> MHQVDPNLTRRKGRLAALAIAAMASASLVTVAVPATANADPEPAPPVPTTAASPPSTAAAPPAPATPVAPPPPAAANTPNAQPGDPNAAPPPADPNAPPPPVI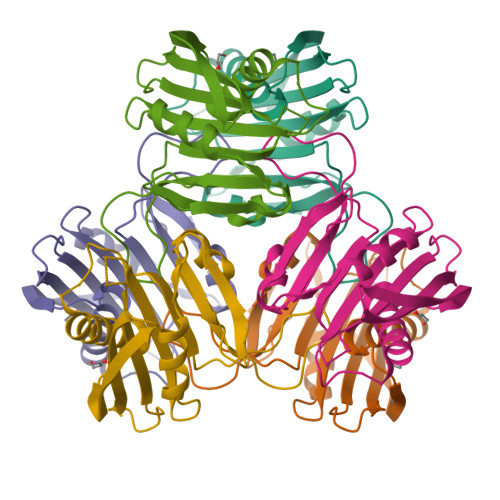APNAPQPVRIDNPVGGFSFALPAGWVESDAAHFDYGSALLSKTTGDPPFPGQPPPVANDTRIVLGRLDQKLYASAEATDSKAAARLGSDMGEFYMPYPGTRINQETVSLDANGVSGSASYYEVKFSDPSKPNGQIWTGVIGSPAANAPDAGPPQRWFVVWLGTANNPVDKGAAKALAESIRPLVAPPPAPAPAPAEPAPAPAPAGEVAPTPTTPTPQRTLPA> ASPEGKVTACHSSQPNATLYKMSSINADFAFNLYRRFTVETPDKNIFFSPVSISAALVMLSFGACCSTQTEIVETLGFNLTDTPMVEIQHGFQHLICSLNFPKKELELQIGNALFIGKHLKPLAKFLNDVKTLYETEVFSTDFSNISAAKQEINSHVEMQTKGKVVG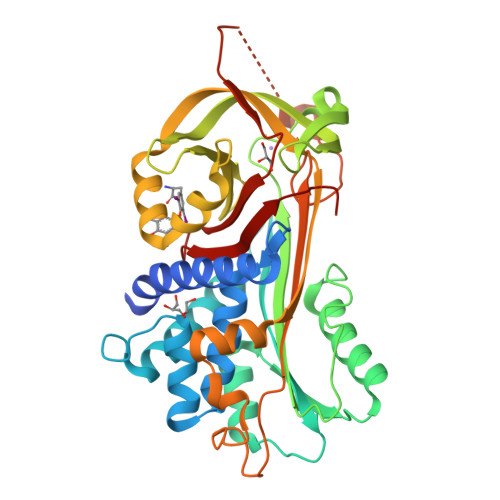LIQDLKPNTIMVLVNYIHFKAQWANPFDPSKTEDSSSFLIDKTTTVQVPMMHQMEQYYHLVDMELNCTVLQMDYSKNALALFVLPKEGQMESVEAAMSSKTLKKWNRLLQKGWVDLFVPKFSISATYDLGATLLKMGIQHAYSENADFSGLTEDNGLKLSNAAHKAVLHIGEKGTEAAAVPEVELSDQPENTFLHPIIQIDRSFMLLILERSTRSILFLGKVVNPTEA>TPYMVQPEYRIYEMNKRLQSRTEDSDNLWWDAFATEFFEDDATLTLSFCLEDGPKRYTIGRTLIPRYFSTVFEGGVTDLYYILKHSKESYHNSSITVDCDQCAMVTQHGKPMFTKVCTEGRLILEFTF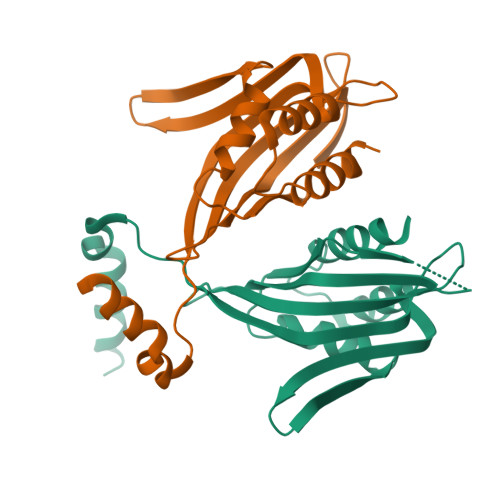DDLMRIKTWHFTIRQYRELVPRSILAMHAQDPQVLDQLSKNITRMGLTNFTLNYLR[2x]>[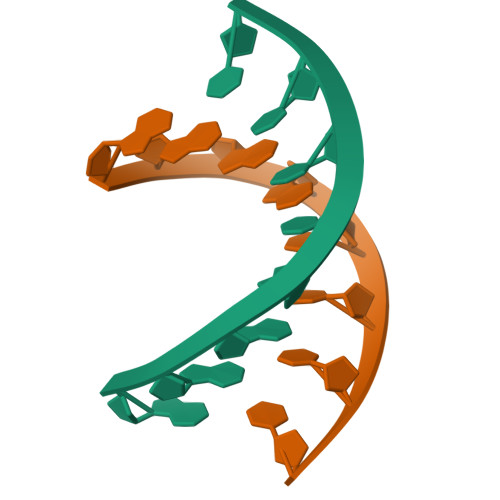2x]GGIGCTCC> AYVEIIEQPKQRGMRFRYKCEGRSAGSIPGERSTDTTKTHPTIKINGYTGPGTVRISLVTKDPPHRPHPHELVGKDCRDGYY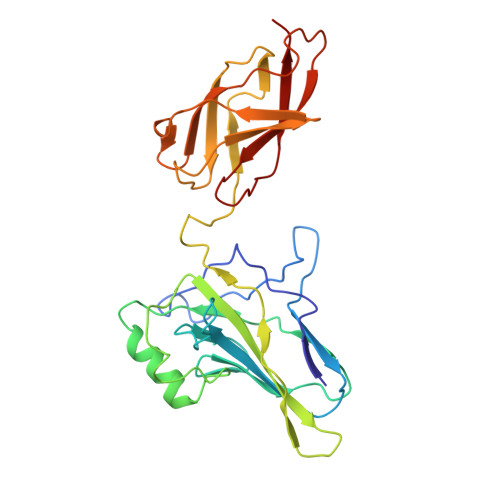EADLCPDRSIHSFQNLGIQCVKKRDLEQAISQRIQTNNNPFHVPIEEQRGDYDLNAVRLCFQVTVRDPAGRPLLLTPVLSHPIFDNRAPNTAELKICRVNRNSGSCLGGDEIFLLCDKVQKEDIEVYFTGPGWEARGSFSQADVHRQVAIVFRTPPYADPSLQAPVRVSMQLRRPSDRELSEPMEFQYLPD> GEIEFIESSKDAGFPVINTPSKTKLEPSVFHQVFEGNKEPAVLRSGDPRLKANFEEAIFSKYIGNVNTHVDEYMLEAVDHYAGQLATLDISTEPMKLEDAVYGTEGLEALDLTTSAGYPYVALGIKKRDILSKKTKDLTKLKECMDKYGLNLPMVTYVKDELRSIEKVAKGKSRLIEASSLNDSVAMRQTFGNLYKTFHLNPG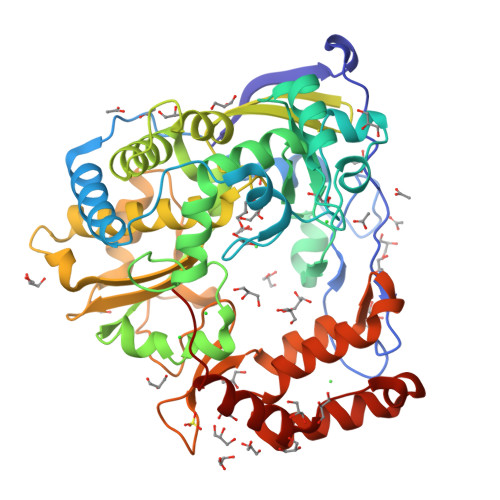VVTGSAVGCDPDLFWSKIPVMLDGHLIAFDYSGYDASLSPVWFACLKMLLEKLGYTHKETNYIDYLCNSHHLYRDKHYFVRGGMPSGCSGTSIFNSMINNIIIRTLMLKVYKGIDLDQFRMIAYGDDVIASYPWPIDASLLAEAGKGYGLIMTPADKGECFNEVTWTNATFLKRYFRADEQYPFLVHPVMPMKDIHESIRWTKDPKNTQDHVRSLCLLAWHNGEHEYEEFIRKIRSVPVGRCLTLPAFSTLRRKWLDSFHHHHHH(3R)-piperidin-3-yl(piperidin-1-yl)methanone | C11 H20 N2 O | 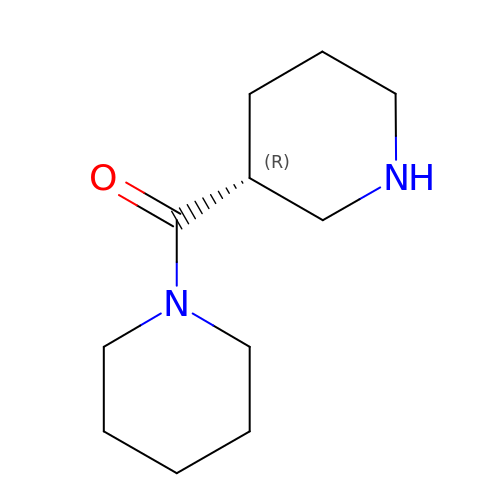OSZRYTYCKGZYLB-SNVBAGLBSA-N>MHHHHHHSAGENLYFQGKEWQENKSWNAHFTEHKSQGVVVLWNENKQQGFTNNLKRANQAFLPASTFKIPNSLIALDL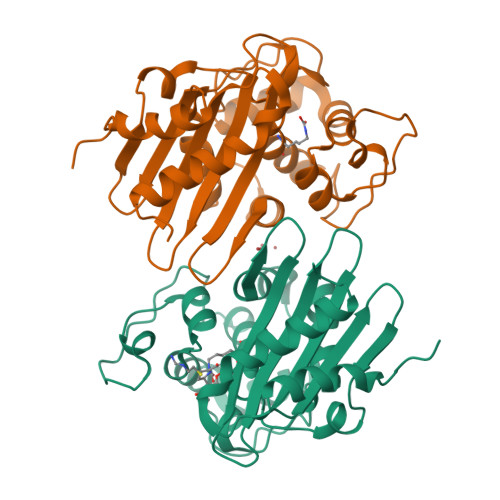GVVKDEHQVFKWDGQTRDIATWNRDHNLITAMKYSVVPVYQEFARQIGEARMSKMLHAFDYGNEDISGNVDSFWLDGGIRISATEQISFLRKLYHNKLHVSERSQRIVKQAMLTEANGDYIIRAKTGYSTRIEPKIGWWVGWVELDDNVWFFAMNMDMPTSDGLGLRQAITKEVLKQEKIIP[4x]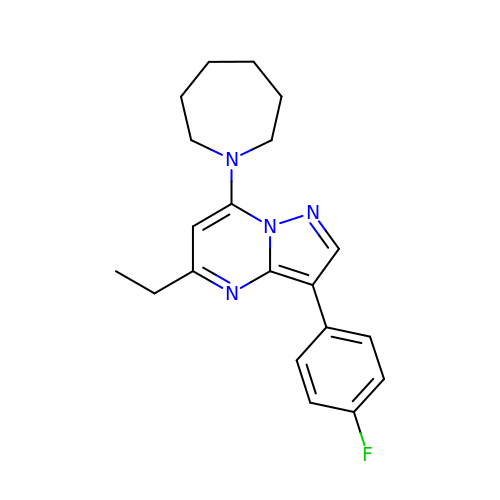7-(azepan-1-yl)-5-ethyl-3-(4-fluorophenyl)pyrazolo[1,5-a]pyrimidine | C20 H23 F N4 | BQIPJVLJUIILIA-UHFFFAOYSA-N> MENKNGGYLPEEEIPDQPPATGAFNYGEALQKAIFFYECQRSGKLDSSTLRLNWRGDSGLDDGKDAGIDLTGGWYDAGDHVKFNLPMSYSAAMLGWAVYEYEDAFKQSGQYNHILNNIKWACDYFIKCHPEKDVYYYQVGDGHADHAWWGPAEVMPMERPSYKVDRSSPGSTVVAETSAALAIASIIFKKVDGEYSKECLKHAKELFEFADTTKSDDGYTAANGFYNSWSGFYDELSWAAVWLYLATNDSSYLDKAESYSDKWGYEPQTNIPKYKWAQCWDDVTYGTYLLLARIKNDNGKYKEAIERHLDWWTTGYNGERITYTPKGLAWLDQWGSLRYATTTAFLACVYSDWENGDKEKAKTYLEFARSQADYAL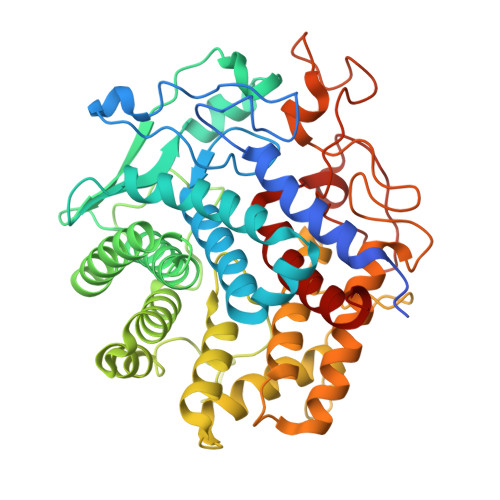GSTGRSFVVGFGENPPKRPHHRTAHGSWADSQMEPPEHRHVLYGALVGGPDSTDNYTDDISNYTCNEVACDYNAGFVGLLAKMYKLYGEL> GPLGSRLEQYEIHI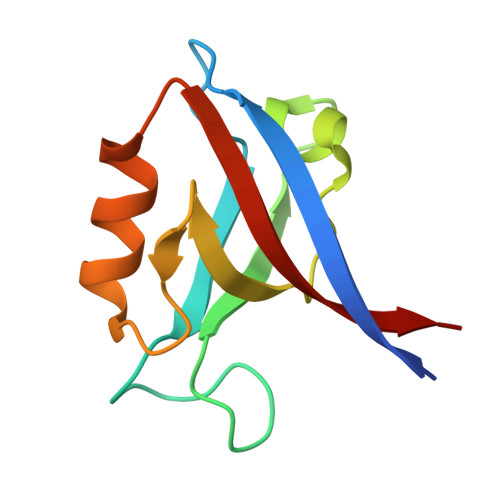ERTAAGLGLSIAGGKGSTPFKGDDDGIFISRVTEAGPADLAGLKVGDKVIKVNGIVVVDADHYQAVQVLKACGAVLVLVVQREVTR>[3x]MNQNLLVTKRDGSTERINLDKIHRVLDWAAEGLHNVSISQVELRSHIQFYDGIKTSDIHETIIKAAADLISRDAPDYQYLAARLAIFHLRKKAYGQFEPPALYDHVVKMVEMGKYDNHLLEDYTEEEFKQMDTFIDHDRDMTFSYAAVKQLEGKYLVQNRVTGEIYESAQFLYILVAACLFSNYPRETRLQYVKRFYDAVSTFKISLPTPI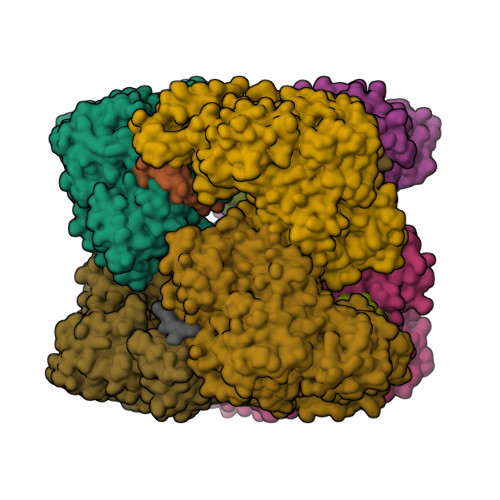MSGVRTPTRQFSSCVLIECGDSLDSINATSSAIVKYVSQRAGIGINAGRIRALGSPIRGGEAFHTGCIPFYKHFQTAVKSCSQGGVRGGAATLFYPMWHLEVESLLVLKNNRGVEGNRVRHMDYGVQINKLMYTRLLKGEDITLFSPSDVPGLYDAFFADQEEFERLYTKYEKDDSIRKQRVKAVELFSLMMQERASTGRIYIQNVDHCNTHSPFDPAIAPVRQSNLALEIALPTKPLNDVNDENGEIALCTLSAFNLGAINNLDELEELAILAVRALDALLDYQDYPIPAAKRGAMGRRTLGIGVINFAYYLAKHGKRYSDGSANNLTHKTFEAIQYYLLKASNELAKEQGACPWFNETTYAKGILPIDTYKKDLDTIANEPLHYDWEALRESIKTHGLRNSTLSALMPSETSSQISNATNGIEPPRGYVSIKASKDGILRQVVPDYEHLHDAYELLWEMPGNDGYLQLVGIMQKFIDQSISANTNYDPSRFPSGKVPMQQLLKDLLTAYKFGVKTLYYQNTRDGAEDAQDDLVPSIQDDGCESGACKI;>YLVGQIDSEVDTDDLSNFQL[4x]> SIITKSIVNADAEARYLSPGELDRIKSFVLSGQRRLRIAQILTDNRELIVKQGGQQLFQKRPDVVSPGGNAYGEEMTATCLRDLDYYLRLVTYGIVAGDVTPIEEIGLV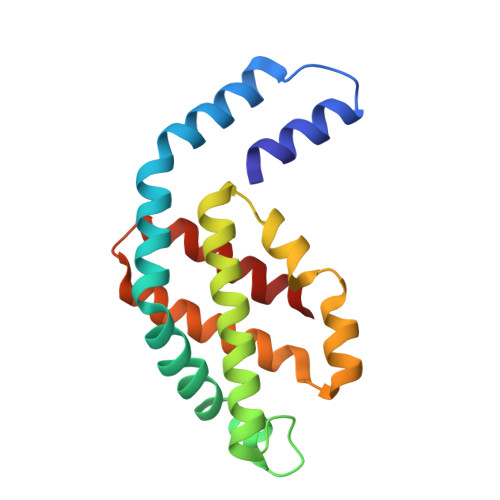GVKEMYNSLGTPISGVAEGVRSMKNVACSLLAGEDSAEAGFYFDYTLGAMQ> MSRKKMGLLVMAYGTPYKEEDIERYYTHIRRGRKPEPEMLQDLKDRYEAIGGISPLAQITEQQAHNLEQHLNEIQDEITFKAYIGLAHIEPFIEDAVAEMHKDGITEAVSIVLAPHFSTFSVQSYNKRAKEEAEKLGGLTITSVESWYDEPKFVTYWVDRVKETYASMPEDERENAMLIVSAHSLPEKIKEFGDPYPDQLHESAKLIAEGAGVSEYAVGWQSEGNTPDPWLGPDVQDLTRDLFEQKGYQAFVYVPVGFVADHLEVLYDNDYECKVVTDDI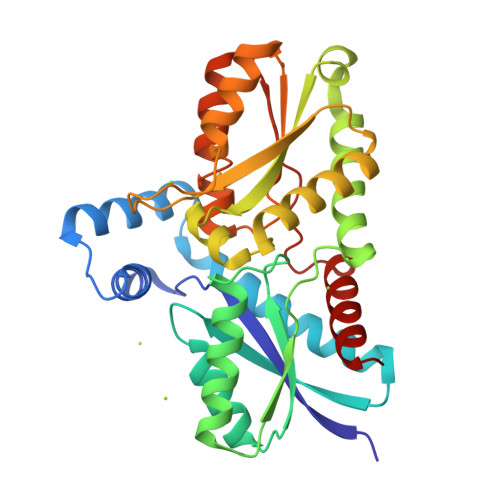GASYYRPEMPNAKPEFIDALATVVLKKLGR> MVTFMITSALHRAADWAKSVFSSAALGDPRRTARLVNVAAQLAKYSGKSITISSEGSKAAQEGAYRFIRNPNVSAEAIRKAGAMQTVKLAQEFPELLAIEDTTSLSYRHQVAEELGKLGSIQDKSRGWWVHSVLLLEATTFRTVGLLHQEWWMRPDDPADADEKESGKWLAAAATSRLRMGSMMSNVIAVCDREADIHAYLQDKLAHNERFVVRSKHPRKDVESGLYLYDHLKNQPELGGYQISIPQKGVVDKRGKRKNRPARKASLSLRSGRITLKQGNITLNAVLAEEINPPKGETPLKWLLLTSEPVESLAQALRVIDIYTHRWRIEEFHKAWKTGAG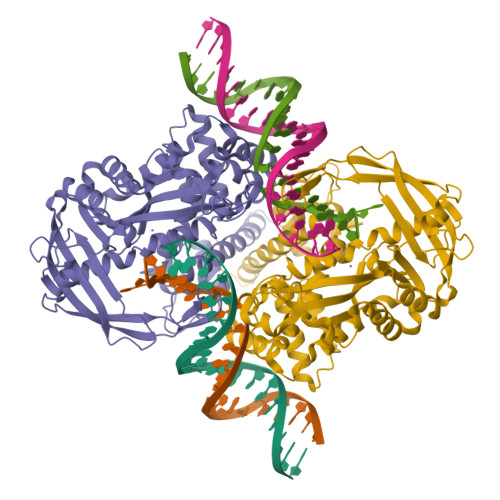AERQRMEKPDNLERMVSILSFVAVRLLQLRESFTPPQALRAQGLLKEAEHVESQSAETVLTPDECQLLGYLDKGKRKRKEKAGSLQWAYMAIARLGGFMDSKRTGIASWGALWEGWEALQSKLDGFLAAKDLMAQGIKIG> GPVTSSLSAEEAQLKVWIQSQIHPRELFGVLSLGKRAAKLDDNPDFVQWLRLVKDFRANNGNQAFSDLDIYYLLLKTNSPEQLKLLFETLRHTPGMTKIGASMEKSLSGNWIRKALEQDTYPTIVYNTLRLKDAGTKLDDTPMFRQWLEYVEKYWNKNAGAFFGDTQMLTLFQKTMTEEEDIIKLVHMLRNNPGMKSHADKLERYLLLT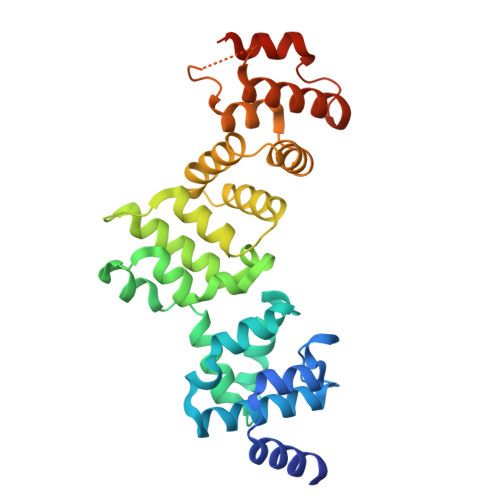SESSHKTMADVWLKARETPEEVFRILRLAEKQTAAADDNRMLNLWLRYTQTYRDKIDKNAFSDAEALQFFRKAKPLDFDWEIV>MVGLLPITAALAATVLPNIVSAVGLDQAAVAKGLQYFGTATDNPELTDIPYVTQLNNTADFGQITPGNSMKWDATEPSQGTFTFTKGDVIADLAEGNGQYLRCHTLVWYNQLPSWVTSGTWTNATLTAALKNHITNVVSHYKGKCLHWDVVNEALNDDGTYRTNIFYTTIGEAYIPIAFAAAAAADPDAKLFYNDYNLEYGGAKAASA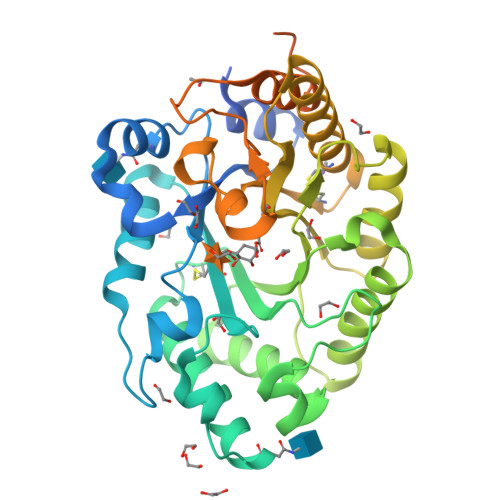RAIVQLVKNAGAKIDGVGLQAHFSVGTVPSTSSLVSVLQSFTALGVEVAYTEADVRILLPTTATTLAQQSSDFQALVQSCVQTTGCVGFTIWDWTDKYSWVPSTFSGYGAALPWDENLVKKPAYNGLLAGMGVTVTTTTTTTTATATGKTTTTTAGAASTGTTAAHWGQCGGLNWSGPTVCASGYTCTYVNDYYSQCL[2x]>[4x]MNVESKWLED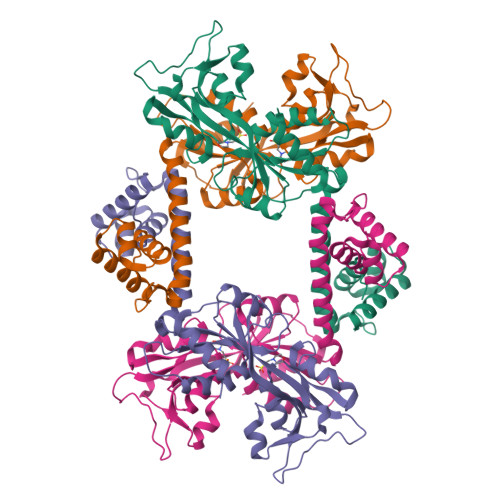FLVLAKVKNFSQAAELRNVTQPAFSRRIRLLEDTVGAELVDRKSKPIELTPSGKLFRITARTLVNQIEAGISQISDLSQLGGNVVQVAAAHSLATSLIPKMQQAFDEGDYKPILSVEAIDVDEATKELREGACDILLAFDDDILRLPPYQSQLIAKTELLPVSACDEMGKPIYDFISQGAVPWLTYSSTSYMGRQVEIIREQVALTPIFSSSMTDMLKILVLNKQGIAWLPAYSIQEELAQKKVAIIGEQSLRLPIEYYAYRYQARLHPAGEKVWSILCNLDT>[4x]CLKEGGDSNSEKFIVGTNATYPPFEFVDKRGEVVGFDIDLAREISNKLGKTLDVREFSFDALILNLKQHRIDAVIT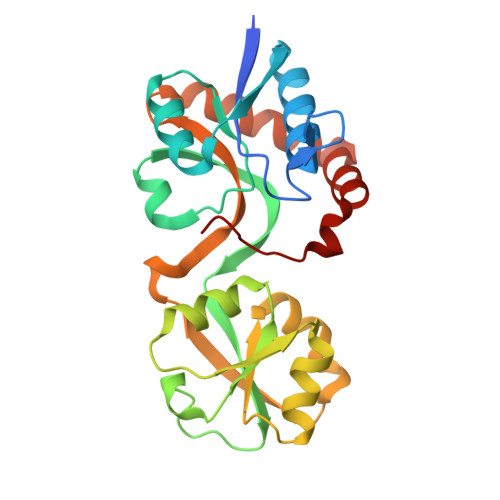GMSITPSRLKEILMIPYYGEEIKHLVLVFKGENKHPLPLTQYRSVAVQTGTYQEAYLQSLSEVHIRSFDSTLEVLMEVMHGKSPVAVLEPSIAQVVLKDFPALSTATIDLPEDQWVLGYGIGVASDRPALALKIEAAVQEIRKEGVLAELEQKWGLNNLEHHHHHH>[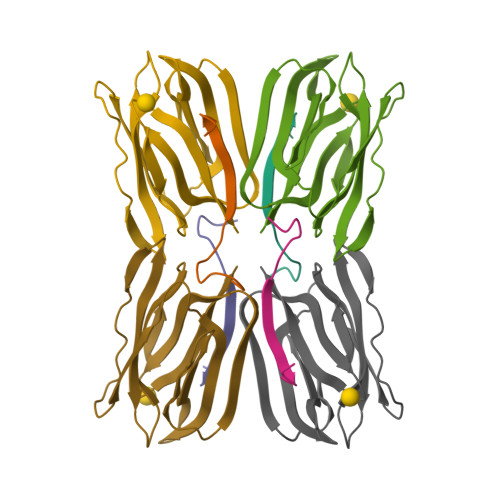4x]AEQSGKSQTVIVGPWGAQV;>[4x]STSSNGKAFDDGAFTGIREINLSYNKETAIGDFQVIYDLNGSPFVGQNHTSFITGFTPVKISLDFPSEYIIEVSGHTGKVSGYVVVRSLAFKTNKKTYGPYGVTSGTPFNLPIENGLIVGFKGSIGYWLDYFSMYLSL> ARTVVLITGCSSGIGLHLAVRLASDPSQSFKVYATLRDLKTQGRLWEAARALACPPGSLETLQLDVRDSKSVAAARERVTEGRVDVLVCNAGLGLLGPLEALGEDAVASVLDVNVVGTVRMLQAFLPDMKRRGSGRVLVTGSVGGLMGLPFNDVYCASKFALEGLCESLAVLLLPFGVHLSLIECGPVHTAFMEKVLGSPEEVLDRTDIHTFHRFYQYLAHSKQVFREAAQNPEEVAEVFLT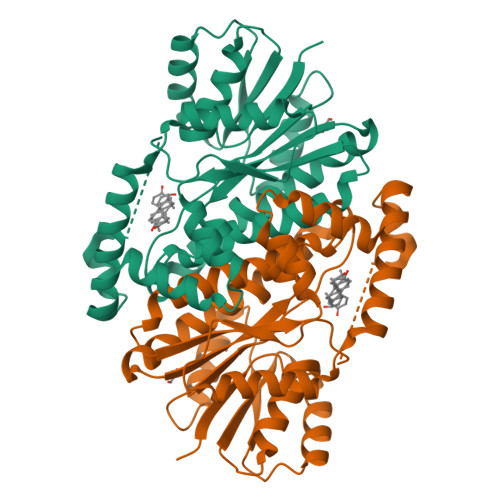ALRAPKPTLRYFTTERFLPLLRMRLDDPSGSNYVTAMHREVFGDVPAKAEAGAEAGGGRGPGAEDEAGRSAVGDPELGDPPAAPQ>[2x]SGISLDNSYKMDYPEMGLCIIINNKNFHKSTGMTSRSGTDVDAANLRETFRNLKYEVRNKNDLTREEIVELMRDVSKEDHSKRSSFVCVLLSHGEEGIIFGTNGPVDLKKITNFFRGDRCRSLTGKPKLFIIQACRGTELDCGIETD;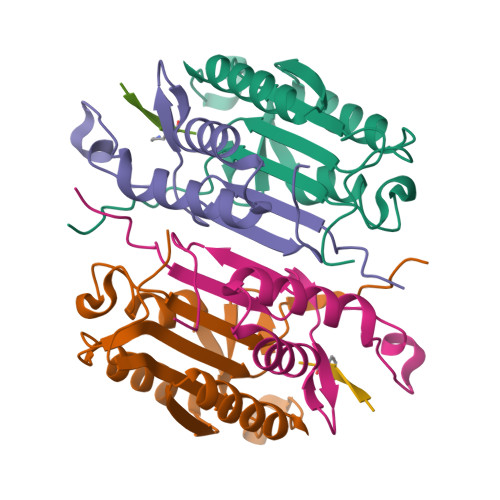>SGVDDDMACHKIPVEADFLYAYSTAPGYYSWRNSKDGSWFIQSLCAMLKQYADKLEFMHILTRVNRKVATEFESFSFDATFHAKKQIPCIVSMLTKELYFYH[2x];>ITVAD[2x]>QGHLRSGPRIFAVWKGHVGQDRVDFGQTEPHTVLFHEPGSSSVWVGGRGKVYLFDFPEGKNASVRTVNIGSTKGSCLDKRDCENYITLLERRSEGLLACGTNARHPSCWNLVNGTVVPLGEMRGYAPFSPDENSLVLFEGDEVYSTIRKQEYNGKIPRFRRIRGESELYTSDTVMQNPQFIKATIVHQDQAYDDKIYYFFREDNPDKNPEAPLNVSRVAQLCRGDQGGESSLSVSKWNTFLKAMLVCSDAATNKNFNRLQDVFLLPDPSGQWRDTRVYGVFSNPWNYSAVCVYSLGDIDKVFRTSSLKGYHSSLPNPRPGKCLPDQQPIPTETFQVADRHPEVAQRVEPMGPLKTPLFHSKYHYQKVAVHRMQASHGETFHVLYLTTDRGTIHKVVEPGEQEHSFAFNIMEIQPFRRAAAIQTMSLDAERRKLYVSSQWEVSQVPLDLCEVYGGGCHGCL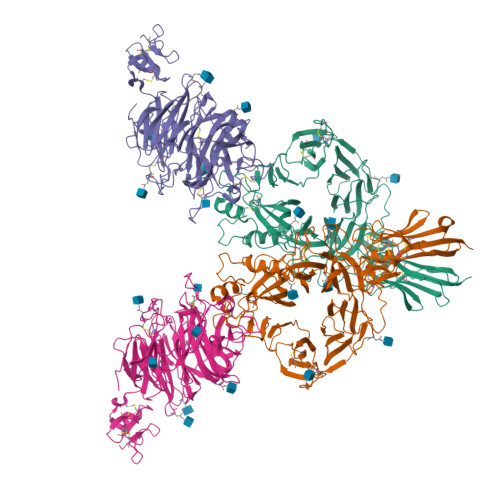MSRDPYCGWDQGRCISIYSSERSVLQSINPAEPHKECPNPKPDKAPLQKVSLAPNSRYYLSCPMESRHATYSWRHKENVEQSCEPGHQSPNCILFIENLTAQQYGHYFCEAQEGSYFREAQHWQLLPEDG[2x];>[2x]ADEPVWRSEQAIGAIAASQEDGVFVASGSCLDQLDYSLEHSLSRLYRDQAGNCTEPVSLAPPARPRPGSSFSKLLLPYREGAAGLGGLLLTGWTFDRGACEVRPLGNLSRNSLRNGTEVVSCHPQGSTAGVVYRAGRNNRWYLAVAATYVLPEPETASRCNPAASDHDTAIALKDTEGRSLATQELGRLKLCEGAGSLHFVDAFLWNGSIYFPYYPYNYTSGAATGWPSMARIAQSTEVLFQGQASLDCGHGHPDGRRLLLSSSLVEALDVWAGVFSAAAGEGQERRSPTTTALCLFRMSEIQARAKRVSWDFKTAESHCKEGDQPERVQPIASSTLIHSDLTSVYGTVVMNRTVLFLGTGDGQLLKVILGENLTSNCPEVIYEIKEETPVFYKLVPDPVKNIYIYLTAGKEVRRIRVANCNKHKSCSECLTATDPHCGWCHSLQRCTFQGDCVHSENLENWLDISSGAKKCPGAP> TCGGCG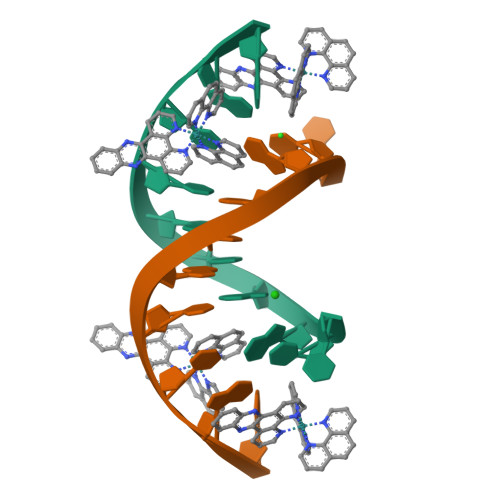CCGA> MGHHHHHHADDDDKDGVDKLSNPFAYLAEPLDPAQPGKKFFNLNKLDYSRYGRLPFSIRVLLEAAVRNCDKFLVKKEDIENILNWNVTQHMNIEVPFKPARVILQDFTGVPSVVDFAAMRDAVKKLGGDPEKINPICPVDLVIDHSIQVDFNRRADSLQKNQDLEFERNRERFEFLKWGSKAFRNMRIIPPGSGIIHQVNLEYLARVVFDQDGYYYPDSLVGTDSHTTMIDGLGVLGWGVGGIEAEAVMLGQPISMVLPQVIGYRLMGKPHPLVTSTDIVLTITKHLRQVGVVGKFVEFFGPGVAQLSIADRATIANMCPEYGATATFFPVDEVSIKYLVQTGRDESKVKQIRKYLQAVGMFRDYSDPSQDPDFTQVVELDLKTVVPCCSGPKRPQDKVAVSDMKKDFESCLGAKQGFKGFQVAPDHHNDHKTFIYNDSEFTLSHGSVVIAAITSSTNTSNPSVMLGAGLLAKKAVDAGLNVKPYVKTSLSPGSGVVTYYLRESGVMPYLSQLGFDVVGYGSMTCIGNSGPLPEPVVEAITQGDLVAVGVLSGNRNFEGRVHPNTRANYLASPPLVIAYAIAGTIRIDFEKEPLGTNAKGQQVFLRDIWPTREEIQAVERQYVIPGMFTEVYQKIETVNASWNALAAPSDKLYLWNPKSTYIKSPPFFENLTLDLQPPKSIVDAYVLLNLGDSVTTDHISPAGNIARNSPAARYLTNRGLTPREFNSYGSRRGNDAIMARGTFANIRLLNRFLNKQAPQTIHLPSGETLDVFDAAERYQQEGHPLIVLAGKEYGSGSSRDWAAKGPFLLGIKAVLAESYERIHRSNLVGMGVIPLEYLPGENADSLGL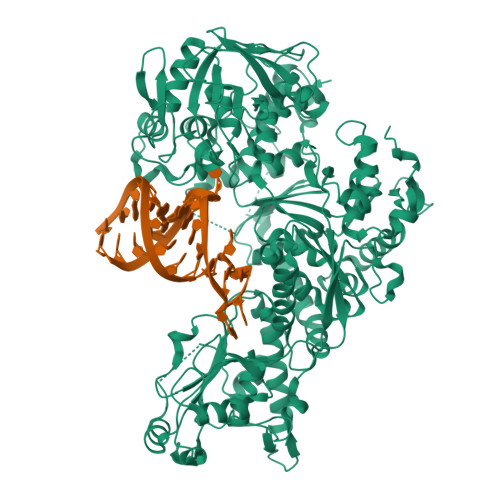TGRERYTIIIPENLTPRMHVQVKLDTGKTFQAVIRFDTDVELTYFHNGGILNYMIRKMAK>[6x]MSDPNADRPPVTVVGLGLMGQALAAAFLKGGHPTTVWNRSPEKAERLVADGAVLADTLESAVTASPLVIVCVSDYDAVHELIRPVESALAGRVLVNLTTATSTQARETAEWAAQRNIPYLDGAIMAIPPVIGTDGAVLLYSGHKSAFEAHESTLKAIAPAATTYLEEDHGLSSLYDMALLGIMWGILNGFLHGAALLGTAKVKAETFAPLANTMISAITEYVTAYAPQVDEGRYEATDATMTVHQAAMEHLAEESEHLGIHSELPRFFKTLADRAVADGHAENSYAAMIELFRKPTA

Recently, C=C bonds conjugated to C=N bonds have been shown to undergo full reduction to amines through the combination of ene-reductases (EREDs) and imine reductases (IREDs),6 as well as the newly discovered ene imine reductase (EneIREDs). The key step involves a stereoselective one-pot amine oxidase/ene imine reductase cascade to convert N-substituted tetrahydropyridines to stereo-defined 3- and 3,4-substituted piperidines. Depending on the EneIRED employed (Series A or B), the kinetic selective reduction of one enantiomer of chiral iminium 3f affords the enantioenriched piperidine 3c as the final product via reduction with a second molecule NADPH (Cycle 2; step vii). Predominantly, EneIREDs in Series A yielded (R)-piperidines whilst enzymes in Series B such as EneIRED-07 yielded the (S)-product.

In order to gain insight into the mode of substrate binding in the active site, we determined the structure of EneIRED-07 from Micromonospora sp. Rc5 to a resolution of 2.55 Å in complex with NADP+ using X-ray crystallography. Crystals were obtained in the P21212 space group and featured six molecules in the asymmetric unit, representing three dimers. EneIRED-07 displays the canonical fold observed for IREDs,38,39 with two monomers associating to form two active sites between the N-terminal Rossmann domain of one subunit and the C-terminal helical bundle of its neighbor. Following building and refinement of the protein atoms, clear omit density was observed in each active site corresponding to the cofactor NADP+. The iminium intermediate (S)-3f, the preferred enantiomer for EneIRED-07 imine reduction, was modeled into the active site using Autodock Vina. The model suggests that the allyl group of (S)-3f is bound within a hydrophobic pocket formed by methionine residues M125, M183, and M214 at the rear of the active site as shown; the para-bromo-phenyl group projects toward the front of the active site bordered by L180, W184, and the NADP+ cofactor. This ligand conformation places the electrophilic carbon approximately 3.6 Å from the NADP+ pyridinium ring C4 atom, from which hydride is transferred. Modeling of the (R)-enantiomer of 3f places the allyl group at the base of the active site with less favorable interactions with hydrophilic residues Y225 and D238.>HHHHHHFNLPPGNYKKPKLLYCSNGHFLRILPDGTVDGTRDRSDQHI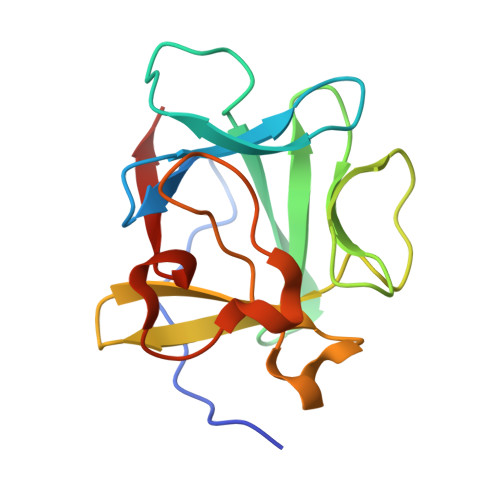QLQLSAESVGEVYIKSTTGQYLAMDTDGLLYGSQTPNEECLFLERLEENHYNTYISKKHAEKNWFVGLKKNGSCKRGPRTHYGQKAILFLPLPVSSD[4x]>AESSVDIQGNDQMQFNTN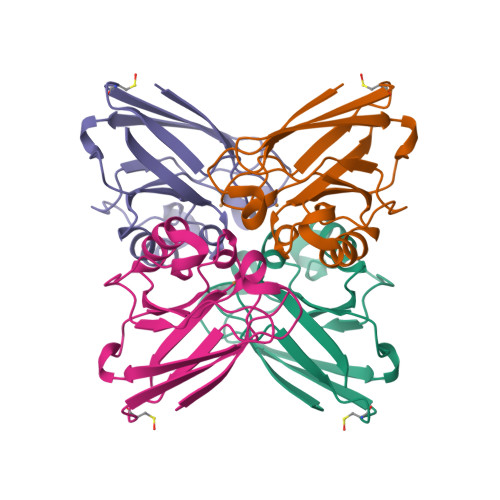AITVDKSCKQFTVNLSHPGNLPKNVMGHNWVLSTAADMQGVVTDGMASGLDKDYLKPDDSRVIAHTKLIGSGEKDSVTFDVPKLKEGEQYMFFCTFPGHSALMKGTLTLK[4x]>[2x]GPYASLTEIEHLVQSVCKSYRETCQLRLEDLLRQRSNIFSREEVTGYQRKSMWEMWERCAHHLTEAI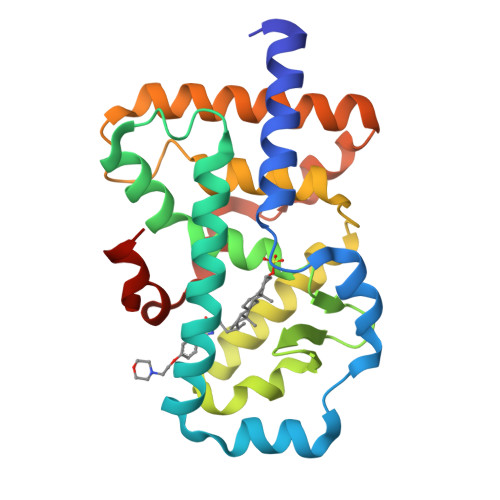QYVVEFAKRLSGFMELCQNDQIVLLKAGAMEVVLVRMCRAYNADNRTVFFEGKYGGMELFRALGCSELISSIFDFSHSLSALHFSEDEIALYTALVLINAHRPGLQEKRKVEQLQYNLELAFHHHLSKTHRQSILAKLPPKGKLRSLCSQHVERLQIFQHLHP> SNLWSTRPERVQEGSTVLINGPQFGWYNPAYTYGIGLHGAGFDVVGNTPFAYPIVLFGTNSEIAWGATAGPQDVVDIYQEKLNPSRADQYWFNNAWRTMEQRKERIQVRGQADREMTIWRTVHGPVMQFDYDQGAAYSKKRSWDGY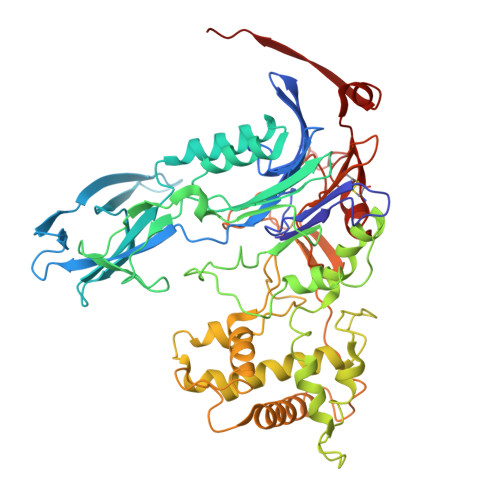EVQSLLAWLNVAKARNWTEFLDQASKMAISINWYYADKHGNIGYVSPAFLPQRPADQDIRVPAKGDGSMEWLGIKSFDAIPKAYNPPQGYLVNWNNKPAPDKTNTDTYYWTYGDRMNELVSQYQQKDLFSVQEIWEFNQKASYSDVNWRYFRPHLEKLAQQLPADDSSKAALTMLLAWDGMEQDQGGQNAGPARVLFKTWLEEMYKQVLMPVVPESHRAMYSQTGFATQQGPNPGSINLSMGTKVLLRALVLEAHPDPKRVNVFGERSSQEIMHTALQNAQARLSQEQGAQMARWTMPTSVHRFSDKNFTGTPQTMPGNTFAFTGYQNRGTENNRVVFDAKGVEFCDAMPPGQSGFTDRNGVRSPHYEDQLKLYENFECKTMDVTHADIRRNAQSSTMLLIQPQP> MHQPKKRLAKKSWAFLTAALTLGVITGVGGYFLFNQNKQRSSVSNFAYQPKQLSVKHQQAVDETLTPWTWNNNNFSSLKITGENPGSFGLVRSQNDNLNISSVTKNSSDDNLKYLNAVEKYLDGQQNFAIRRYDNNGRALYDINLAKMENPSTVQRGLNGEPIFDPFKGFGLTGNAPTDWNEIKGKVPVEVVQSPHSPNLYFVLLVPKVALEYHNLNNQVVKESLEVKATQSSFNPTQRLQKDSPVKDSSKQGEKLSETTASSMSSGMATSTRAKALKVEVERGSQSDSLLKNDFAKKPLKHKNSSGEVKLEAEKEFTEAWKPLLTTDQIAREKGMGATVVSFYDAPYSENHTAFGLVDHIDPKKMVENYPPSWKTPKWNHHGIWDYNARNLLLQTTGFFNPRRHPEWFDEGQAKADNTSPGFKVGDTDHKKDGFKKNSSSPIALPFEAYFANIGNMVAIGNSVFIFGGNGHATKMFTTNPLSIGVFRIKYTDNFSKSSVTGWPYAVLFGGLINPQTNGLKDLPLGTNRWFEYVPRMAVSGVKWVGNQLVLAGTLTMGDTATVPRLKYDQLEKHLNLVAQGQGLLREDLQIFTPYGWANRPDIPVGAWLQDEMGSKFGPHYFLNNPDIQDNVNNDTVEALISSYKNTDKLKHVYPYRYSGLYAWQLFNWSNKLTNTPLSANFVNENSYAPNSLFAAILNEDLLTGLSDKIFYGKENEFAENEADRFNQLLSLNPNPNTNWARYLNVVQRFTTGPNLDSSTFDQFLDFLPWIGNGKPFSNSPSPSTSASSSTPLPTFSNINVGVKSMITQHLNKENTRWVFIPNFSPDIWTGAGYRVQSANQKNGIPFEQVKPSNNSTPFDPNSDDNKVTPSGGSSKPTTYPALPNSISPTSDWINALTFTNKNNPQRNQLLLRSLLGTIPVLINKSGDSNDQFNKDSEQKWDKTETNEGNLPGFGEVNGLYNAALLHTYGFFGTNTNSTDPKIGFKADSSSSSSSTLVGSGLNWTSQDVGNLVVINDTSFGFQLGGWF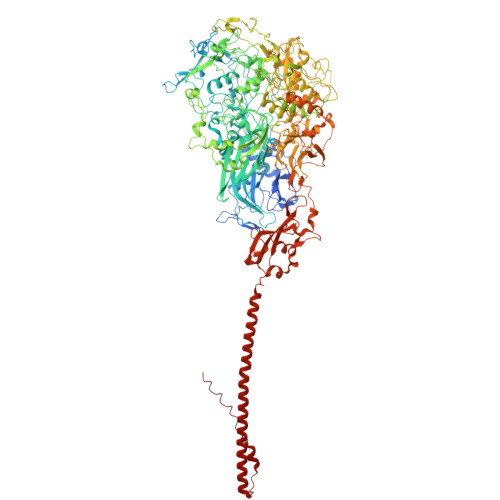ITFTDFIRPRTGYLGITLSSLQDQTIIWADQPWTSFKGSYLDSDGTPKSLWDPTALKSLPNSSTTYDTNPTLSPSFQLYQPNKVKAYQTTNTYNKLIEPVDATSAATNMTSLLKLLTTKNIKAKLGKGTASSQGNNNGGGVSQTINTITTTGNISEGLKEETSIQAETLKKFFDSKQNNKSEIGIGDSTFTKMDGKLTGVVSTPLVNLINGQGATSDSDTEKISFKPGNQIDFNRLFTLPVTELFDPNTMFVYDQYVPLLVNLPSGFDQASIRLKVISYSVENQTLGVRLEFKDPQTQQFIPVLNASSTGPQTVFQPFNQWADYVLPLIVTVPIVVIILSVTLGLTIGIPMHRNKKALQAGFDLSNKKVDVLTKAVGSVFKEIINRTGISNAPKKLKQATPTKPTPKTPPKPPVKQ>MNLPDNSIHLQLPRPVCEAIIRPVPEHRADQELSEIYRDLKATFGVPWVGVITQAVAYYRPFFAEAWRRFAPSAKTHFFERASDDIRIRSWELMGQSFVIEGQTDRLREMGYSVREIGQIRAVLDIFDYGNPKYLIFA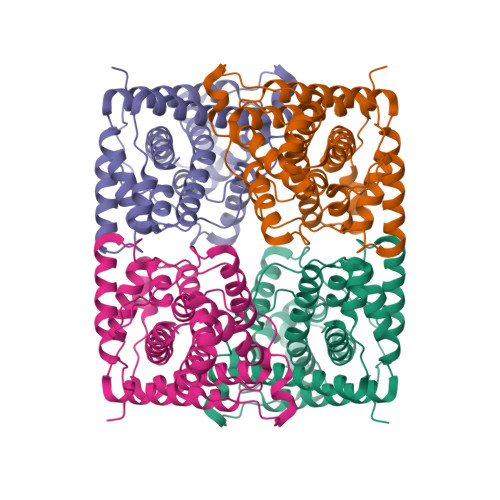TAIKEGLLSGRTFGGAAGDARCHFPRSPICQIDPIPVMVEEHHAGGTLSQVYADIKQTLQLPFINSDYKAMARWPSYLEQAWGALKPCIDTPAYQAGRFDINARALAALDALPTAYRMSRDDALQAGLSEAQTDELIQVISLFQWMLSGIVLNVTHFKQQALKLEHHHHHH[4x]> MSDLVNKKFPAGDYKFQYIAISQSDADSESCKMPQTVEWSKLISENKKVIITGAPAAFSPTSTVSHIPGYINYLDELVKEKEVDQVIVVTVDNPFANQAWAKSLGVKDTTHIKFASDPGCAFTKSIGFELAVGDGVYWS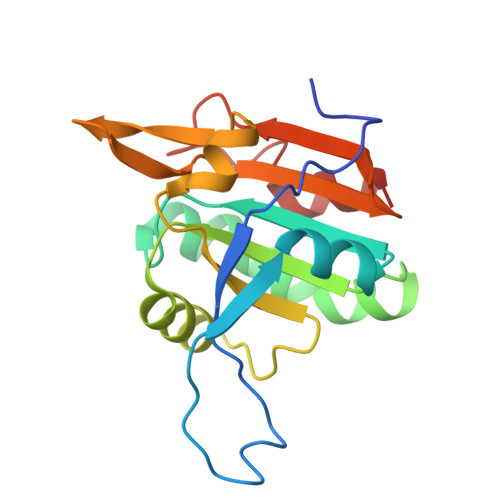GRWAMVVENGIVTYAAKETNPGTDVTVSSVESVLAHL> GPLGSGDVQVTEDAVRRYLTRKPMTTKDLLKKFQTKKTGLSSEQTVN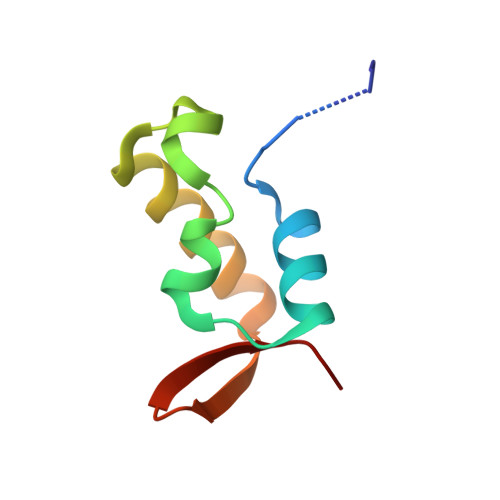VLAQILKRLNPERKMINDKMHFSLKE>PSVYDAAAQLTADVKKDLRDSWKVIGSDKKGNGVALMTTLFADNQETIGYFKRLGDVSQGMANDKLRGHSITLMYALQNFIDQLDNPDDL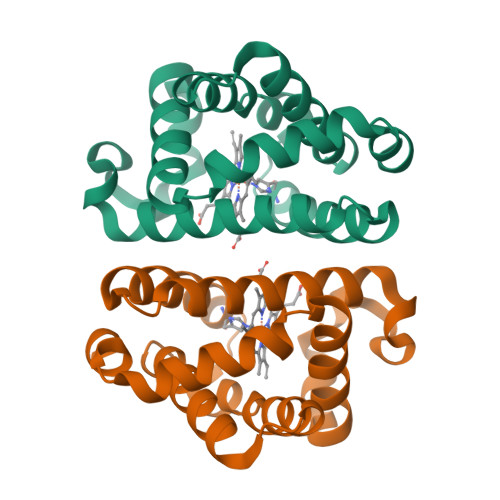VCVVEKLAVNHITRKISAAEFGKINGPIKKVLASKNFGDKYANAWAKLVAVVQAAL[2x]> GSQMTRQARRLYVGNIPFGITEEAMMDFFNAQMRLGGLTQAPGNPVLAVQINQDKNFAFLEFRSVDETTQAMAFDGIIFQGQSLKIRRPHDYQPLPGMSENPSVYVPGVVST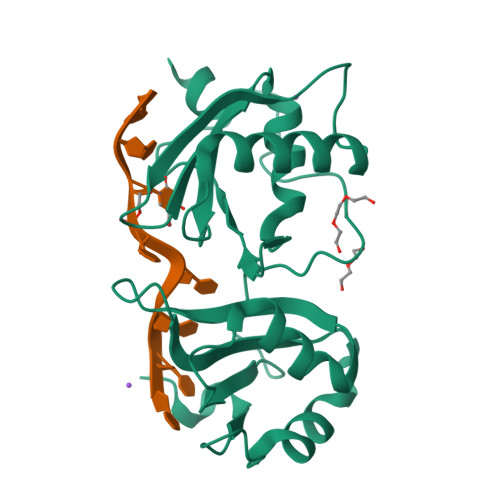VVPDSAHKLFIGGLPNYLNDDQVKELLTSFGPLKAFNLVKDSATGLSKGYAFCEYVDINVTDQAIAGLNGMQLGDKKLLVQRASVGAKN[2-(3-DIBENZOFURAN-4-YL-PHENYL)-1-HYDROXY-1-PHOSPHONO-ETHYL]-PHOSPHONIC 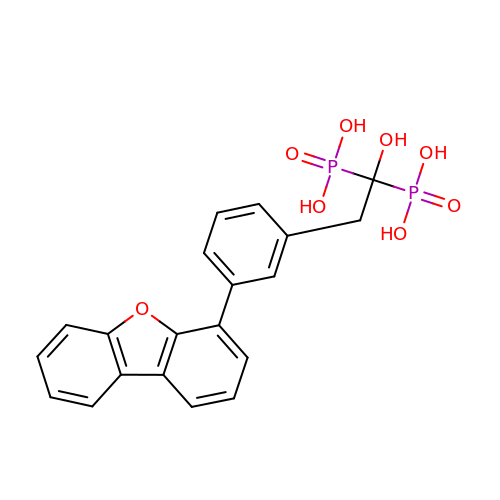ACID | C20 H18 O8 P2 | BYVXAUZOTGITQZ-UHFFFAOYSA-N(5E)-2-azanylidene-5-[(2,3-dimethoxyphenyl)methylidene]-1,3-thiazolidin-4-one | C12 H12 N2 O3 S | 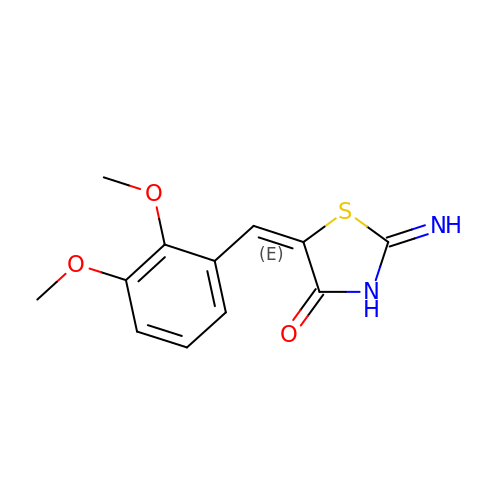GUZXOEURHZVATE-RMKNXTFCSA-N> MDRKISSTRRVRTYPLAPEKAEIFNSMHGWVEDTILPFLKPVEESWQPTDFLPDSTSDGFHEQVEELRKRTADLPDDYLVALVGAMVTEEALPTYQTMLNTTDVIYDESGASPVPWAVWTRAWTAEENRHGDIVNKYLYLSGRVDMKQIEKTIQYLIGSGMDPGADNNPYLAYIYTSYQERATAISHGSLGRLARQKGEMKLAQICGTISADEKRHEAAYSKIVEKLFELDPEGTMLALAYMMKMKIVMPARLMHDGKDPDMFQHFSAVSQRLGIYTAKEYTDILEHMIARWGVDKLTGLSGEGRRAQDYVCGLPMRFRKVEERAQAWAENISHVPFSWIFG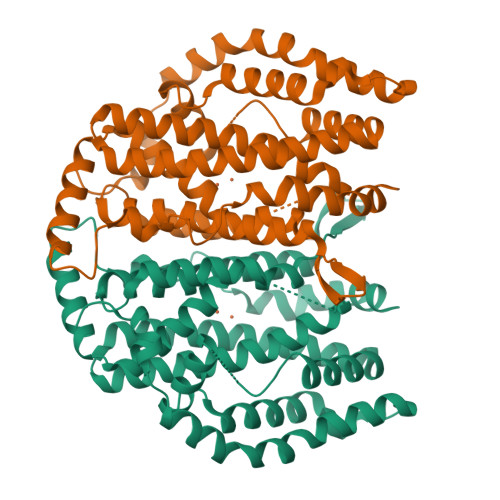RRV> MSMMAERDMGRILLDLSDDVIQRLDDLKVQRNIPRAELLREAVEQYLEKQDRAKDT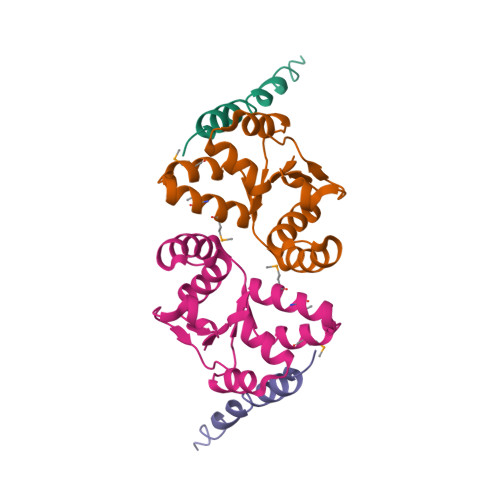ISSALGLWQDCEEDGMEYQRQLRKEW;> MTSGSALFDTNILIDLFSGRREAKQALEAWPPQNAISLITWMEVMVGAKKYHQEQRTRMALSTFNIINISQDIAERSVALRQEYKLKLPDAIILATAQLHRLELITRNTKDFAGIPGVVTPYEIHPE9-(3,5-dichloro-4-hydroxyphenyl)-1-{trans-4-[(dimethylamino)methyl]cyclohexyl}-3,4-dihydropyrimido[5,4-c]quinolin-2(1H)-one 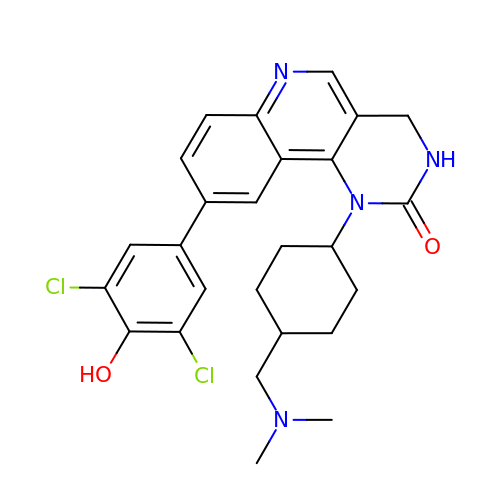| C26 H28 Cl2 N4 O2 | FUVRHGKKWNNBJX-RHDGDCLCSA-N>SATTIQKELENIVVKERQNKKDTILMGLKVEVPWNYCDWASISFYDVRLESGILDMESIAVKYMTGCDIPPHVTLGITNKDQEANFQRFKELTRNIDLTSLSFTCKEVICFPQSRASKELGANGRAVVMKLEASDDVKALRNVLFNVVPTPRDIFGPVLSDPVWCPHVTIGYVRADDEDNKNSFIELAEAFRGSKIKVIGWCE[4x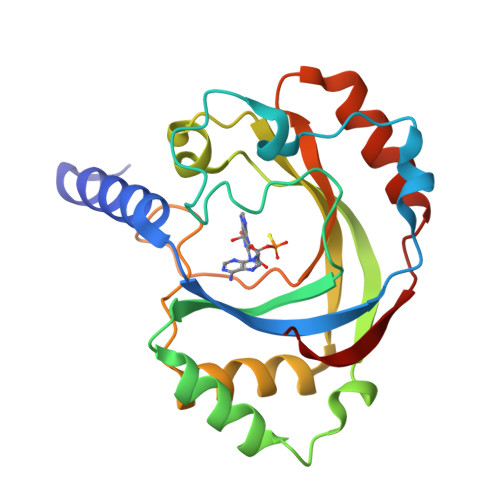]>[3x]RADPGPLQDFCLADLNSPLFINGYPCRNPALATSDDFIYSGFKQAPSGFDQWGLNVTFVTAGQFPALNTLGLTINR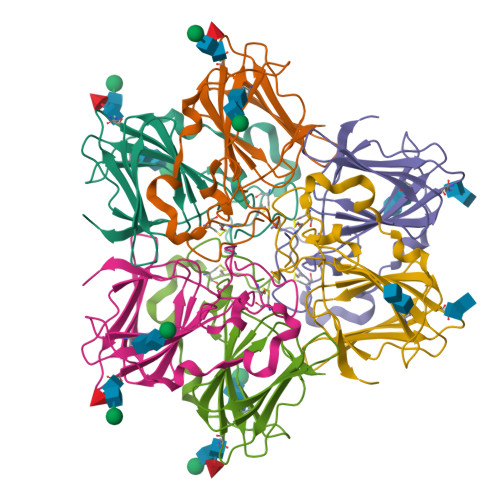CVLLPGGSTQFRTNPRASSLVMATEGEILEGFYSTNDNQLYVKRLTPGDLFIIPPGLMHFTVNVGTGNATFYASLNSQNPGGQIVGLMDETVIAHLKAQYPNVVSQMLPSVNDRINSKIPVIKLPL> MSGSVMLGESS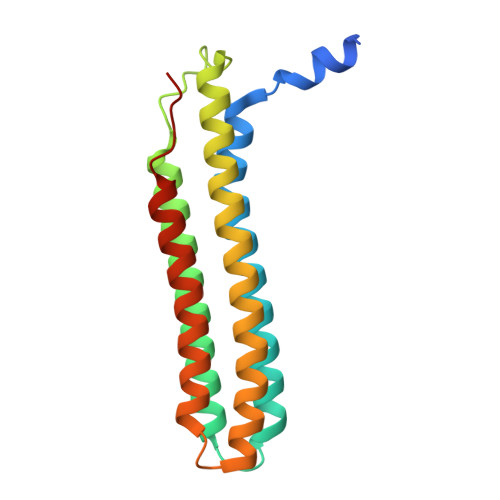SWSRALVKISPYTFSAIGIAVAIGVSVLGAAWGIYITGSSLIGAAIKAPRITSKNLISVIFCEAVAIYGVIVAIILQTKLESVPASQIYAPESLRAGYAIFASGIIVGFANLVCGLCVGIIGSSCALSDAQNSSLFVKILVIEIFGSALGLFGVIVGIIMSAQASWPAKPV>[2x]DEVPELRIEKVKENIFLHTSYSRVNG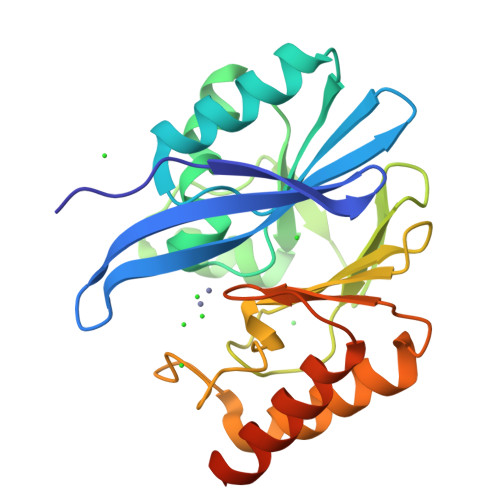FGLVSSNGLVVIDKGNAFIVDTPWSDRDTETLVHWIRKNGYELLGSVSTHWHEDRTAGIKWLNDQSISTYATTSTNHLLKENKKEPAKYTLKGNESTLVDGLIEVFYPGGGHTIDNVVVWLPKSKILFGGCFVRSLDSEGLGYTGEAHIDQWSRSAQNALSRYSEAQIVIPGHGKIGDIALLKHTKSLAETASNKSIQPNANASAD Signaling through RET plays essential regulatory roles in the development of the nervous system and kidney. Glia cell line-derived growth factor (GDNF), Neurturin (NRTN), Artemin (ARTN) and Persephin are four ligands that induce dimerization of RET through assembling 2:2:2 ternary complexes with RET and the co-receptors GDNF receptor-α family proteins (GFRα1–4). Here, we report the cryo-EM structures of four extracellular 2:2:2 ligand/co-receptor/RET complexes, including GDF15/GFRAL/RET, GDNF/GFRα1/RET, NRTN/GFRα2/RET and ARTN/GFRα3/RET, at near-atomic resolution. The structures show that the extracellular region of RET adopts a ‘C-clamp’ shape, which is stabilized by extensive inter-domain interactions as well as binding of calcium ion at multiple sites.

Surprisingly, our cryo-EM results reveal that two 2:2:2 NRTN/GFRα2/RET complexes can dimerize to form a 4:4:4 complex through a novel ligand/receptor interface. With further 3D classification for the dataset of the NRTN/GFRα2/RET complex, we identified one class showing two 2:2:2 complexes arranged in a staggered fashion to form a 4:4:4 complex that resembles a four-bladed propeller. Subsequent 3D refinement yielded a map at 4.3 Å resolution, allowing us to build a complete model of the 4:4:4 complex by rigid-body fitting the atomic models of the protein components into cryo-EM map. The 4:4:4 NRTN/GFRα2/RET complex is mediated by a novel interface, formed between the protruding ‘elbow’ at the CLD4-CRD junction of RET and the convex face of NRTN near the GFRα2-binding site. Particularly, the loop connecting CLD4 and CRD (residues 507–513) in RET makes a number of interactions with the surface of the major β-sheet in NRTN. Several charged residues in NTRN, including Arg101, Arg106, Glu107, Arg128, and Arg155, contribute to the interaction. 3D classification result of this mutant complex clearly showed that the double mutations in NRTN exclusively abolished the formation of the 4:4:4 complex, but not the 2:2:2 complex, verifying that the novel NRTN/RET interface is responsible merely for the formation of the higher-order oligomer. We found that the 4:4:4 complex suppresses RET endocytosis. Our data suggest that the formation of the 4:4:4 NRTN/GFRα2/RET complex delays RET endocytosis, likely leading to more sustained signaling.

>ARLGARPCGLRELEVRVSELGLGYASDETVLFRYCAGACEAAARVYDLGLRRLRQRRRLRRERVRAQPCCRPTAYEDEVSFLDAHSRYHTVHELSARECACV[4x];>[4x]SSLQGPELHGWRPPVDCVRANELCAAESNCSSRYRTLRQCLAGRDRNTMLANKECQAALEVLQESPLYDCRCKRGMKKELQCLQIYWSIHLGLTEGEEFYEASPYEPVTSRLSDIFRLASIFSGTGADPVVSAKSNHCLDAAKACNLNDNCKKLRSSYISICNREISPTERCNRRKCHKALRQFFDRVPSEYTYRMLFCSCQDQACAERRRQTILPSCSYEDKEKPNCLDLRGVCRTDHLCRSRLADFHANCRASYQTVTSCPADNYQACLGSYAGMIGFDMTPNYVDSSPTGIVVSPWCSCRGSGNMEEECEKFLRDFTENPCLRNAIQAFGNGTDVNGTHHHHHHHH;>[4x]LYFSRDAYWEKLYVDQAAGTPLLYVHALRDAPEEVPSFRLGQHLYGTYRTRLHENNWICIQEDTGLLYLNRSLDHSSWEKLSVRNHGFPLLTVYLKVFLSPTSLREGECQWPGCARVYFSFFNTSFPACSSLKPRELCFPETRPSFRIRENRPPGTFHQFRLLPVQFLCPNISVAYRLLEGEGLPFRCAPDSLEVSTRWALDREQREKYELVAVCTVHAGAREEVVMVPFPVTVYDEDDSAPTFPAGVDTASAVVEFKRKEDTVVATLRVFDADVVPASGELVRRYTSTLLPGDTWAQQTFRVEHWPNETSVQANGSFVRATVHDYRLVLNRNLSISENRTMQLAVLVNDSDFQGPGAGVLLLHFNVSVLPVSLHLPSTYSLSVSRRARRFAQIGKVCVENCQAFSGINVQYKLHSSGANCSTLGVVTSAEDTSGILFVNDTKALRRPKCAELHYMVVATDQQTSRQAQAQLLVTVEGSYVAEEAGCPLSCAVSKRRLECEECGGLGSPTGRCEWRQGDGKGITRNFSTCSPSTKTCPDGHCDVVETQDINICPQDCLRGSIVGGHEPGEPRGIKAGYGTCNCFPEEEKCFCEPEDIQDPLCDELCRGTHHHHHHHH>MRGSHHHHHHGMASMAVSESQLK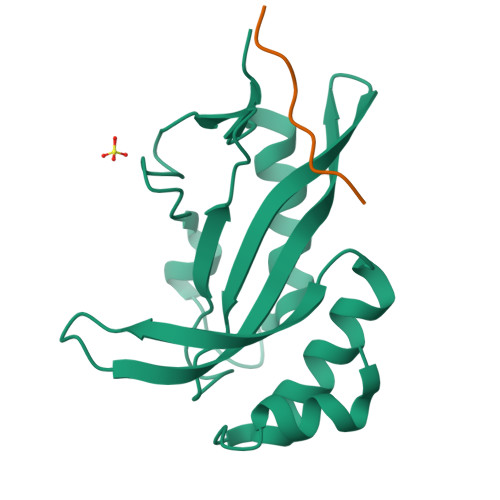KMVSKYKYRDLTVRETVNVITLYKDLKPVLDSYVFNDGSSRELMNLTGTIPVPYRGNTYNIPICLWLLDTYPYNPPICFVKPTSSMTIKTGKHVDANGKIYLPYLHEWKHPQSDLLGLIQVMIVVFGDEPPVFSRP[2x];>ILPTAPPEY[2x]> MKINLSWKTYAVLSIVSLGGIHAMEDVPAELTGVSEGYTRFYRSPTASVTLSGLVNVKWDNEQMTMPLFKWIGGEQAEELHFCVHIAHSIGPKLNLARTLGTVNSNMDQHWAQAHRHSGATRRTIQDFHLFANDIPNFP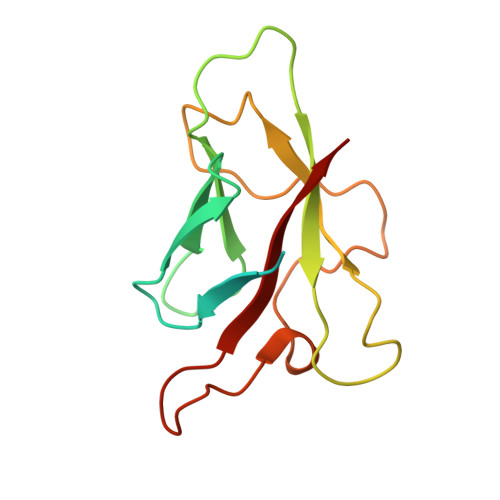DYIKIKLVPKT>GGU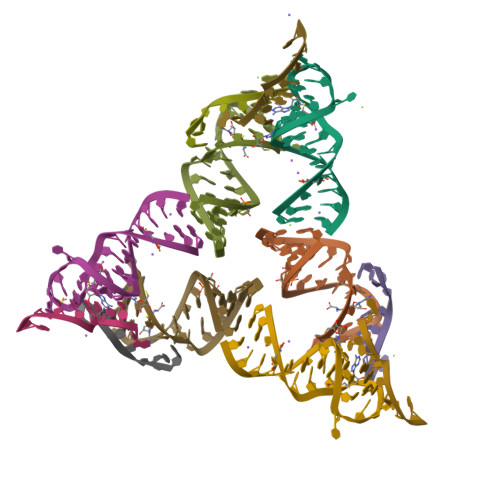CACAACGGCUUCCUGGCGUGACCAUUGGAGCA[12x]~{N}-[5-(azepan-1-ylsulfonyl)-2-methoxy-phenyl]-2-(1~{H}-indol-3-yl)ethanamide | 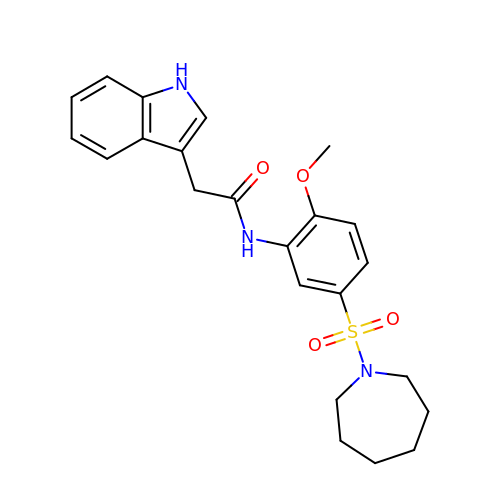C23 H27 N3 O4 S | WUSKETSOXMZDPT-UHFFFAOYSA-N>[6x]GP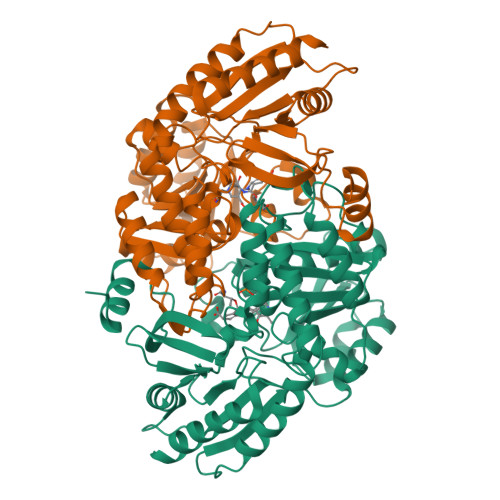PTSDDIFEREYKYGAHNYHPLPVALERGKGIYLWDVEGRKYFDFLSSYSAVNQGHCHPKIVNALKSQVDKLTLTSRAFYNNVLGEYEEYITKLFNYHKVLPMNTGVEAGETACKLARKWGYTVKGIQKYKAKIVFAAGNFWGRTLSAISSSTDPTSYDGFGPFMPGFDIIPYNDLPALERALQDPNVAAFMVEPIQGEAGVVVPDPGYLMGVRELCTRHQVLFIADEIQTGLARTGRWLAVDYENVRPDIVLLGKALSGGLYPVSAVLCDDDIMLTIKPGEHGSTYGGNPLGCRVAIAALEVLEEENLAENADKLGIILRNELMKLPSDVVTAVRGKGLLNAIVIKETKDWDAWKVCLRLRDNGLLAKPTHGDIIRFAPPLVIKEDELRESIEIINKTILSF> GALEDNEHLFQFSCLMQNKHRRVLPIDICNPLTKFNFLECICNCLMTKQSVNVNE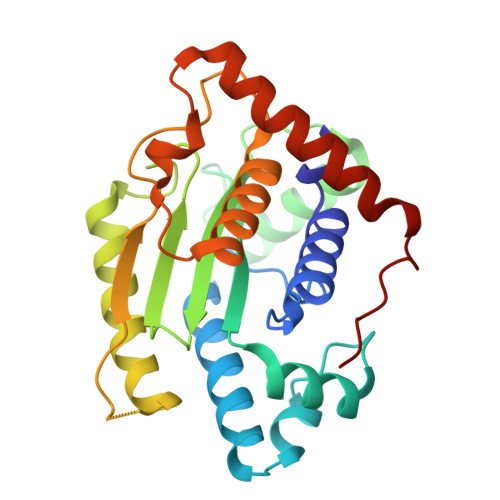TDMCELFCPPTCTPENYRRLLCTSSVFPFVMWHDPSADTQEAMLTKMDQTMSSGRVGNSHWVLVIVDIEYRCVTFFDSLCDYVASPQQMREQLEGLAVSLGAIYPKEGGADSDQEELLSPFQVRIGSTVKVQSPGEFTCGAWCCQFLAWYLENPDFDLEEKVPTNPSERRALLADFISTTEQAMSRYSSLSWPTTD13-diphenylalkyl Berberine | C36 H34 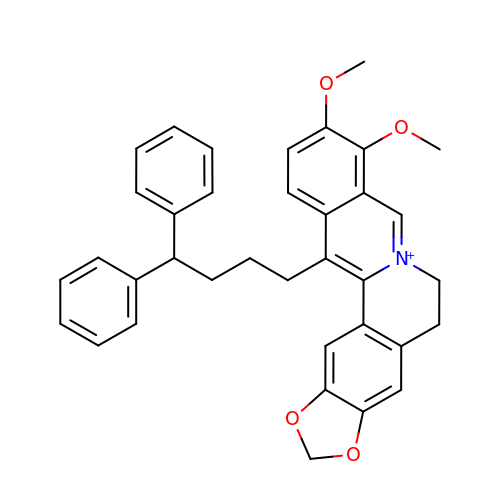N O4 | GTWMZDSMZWCFBR-UHFFFAOYSA-N> MTTTERPDLAWLDEVTMTQLERNPYEVYERLRAEAPLAFVPVLGSYVASTAEVCREVATSPDFEAVITPAGGRTFGHPAIIGVNGDIHADLRSMVEPALQPAEVDRWIDDLVRPIARRYLERFENDGHAELVAQYCEPVSVRSLGDLLGLQEVDSDKLREWFAKLNRSATNAAVDENGEFANPEGFAEGDQAKAEIRAVVDPLIDKWIEHPDDSAISHWLHDGMPPGQTRDREYIYPTIYVYLLGAMQEPGHGMASTLVGLFSRPEQLEEVVDDPTLIPRAIAEGLRWTSPIWSATARISTKPVTIAGVDLPAGTPVMLSYGSANHDTGKYEAPSQYDLHRPPLPHLAFGAGNHACAGIYFANHVMRIALEELFEAIPNLERDTREGVEFWGWGFRGPTSLHVTWEV

GcoA belongs to the CYP255A family of cytochrome P450 enzymes. Our recent characterization of a two-component P450 enzyme system consisting of a reductase, GcoB, and a P450 oxidase, GcoA, demonstrated that it demethylates diverse aromatic compounds, including guaiacol (which can be derived from coniferyl alcohol and represents the aromatic functionality of G-lignin that must undergo demethylation), guaethol, anisole (methoxybenzene), 2-methylanisole, and 3-methoxycatechol (3MC) with similar or greater efficiency than other O-aryl-demethylases described in the literature. However, GcoAB shows poor reactivity toward syringol, which can be derived from sinapyl alcohol via high-temperature reactions and represents the aromatic functionality of S-lignin that must undergo O-demethylation for further catabolism via ring-opening dioxygenases. In the present study, we hypothesized that substitution of GcoA-F169, which has the closest interaction with the bound substrate, may relax the specificity of the enzyme sufficiently to permit the O-demethylation of S-lignin type substrates.

Thus, we prepared the GcoA-F169A variant and measured its guaiacol and syringol binding properties. Both ligands were able to stimulate the Fe(III) spin state conversion at levels close to wild-type (WT), with KD values in the low micromolar range. Each protein variant also crystallized successfully with guaiacol and the structures showed that the orientation of the bound ligand remained consistent with that of the WT enzyme. Even the largest reduction in side chain bulk, represented by the GcoA-F169A variant, retained the ideal reactive geometry for the natural substrate. Furthermore, comparison of the surrounding active site architecture confirmed no significant deviation from the WT. When NADH and O2 were present in excess of guaiacol, the measured stoichiometry of the GcoA-F169A–catalyzed reaction was very close to 1 molecule each of guaiacol and NADH consumed to 1 formaldehyde and 1 catechol produced, without overconsumption of NADH (103 ± 7% coupling efficiency). Moreover, GcoA-F169A has a slightly improved performance with guaiacol as a substrate relative to the WT enzyme. Thus, the GcoA-F169A mutant, which showed enhanced turnover on guaiacol and syringol, is closer to the CYP255A consensus protein than the WT. Unexpectedly, we found that GcoA-F169A not only binds both guaiacol and syringol in a productive orientation analogous to guaiacol in WT GcoA, but also is more catalytically efficient for O-demethylation of both guaiacol and syringol relative to WT, where O-demethylation is well coupled to NADH oxidation.> MAEKSIFNEPDVDFHLKLNQQLFHIPYELLSKRIKHTQAVINKETKSLHEHTAALNQIFEHNDVEHDELALAKITEMIRKVDHIERFLNTQIKSYCQILNRIKKRLEFFHELKDIKSQNSGTSHNGNNEGTRTKLIQWYQSYTNILIGDYLTRNNPIKYNSETKDHWNSGVVFLKQSQLDDLIDYDVLLEANRISTSLLHERNLLPLISWINENKKTLTKKSSILEFQARLQEYIELLKVDNYTDAIVCFQRFLLPFVKSNFTDLKLASGLLIFIKYCNDQKPTSSTSSGFDTEEIKSQSLPMKKDRIFQHFFHKSLPRITSKPAVNTTDYDKSSLINLQSGDFERYLNLLDDQRWSVLNDLFLSDFYSMYGISQNDPLLIYLSLGISSLKTRDCLHPSDDENGNQETETATTAEKEVEDLQLFTLHSLKRXXXXXXXXXXXXXXXXXXXXXXXXXXXX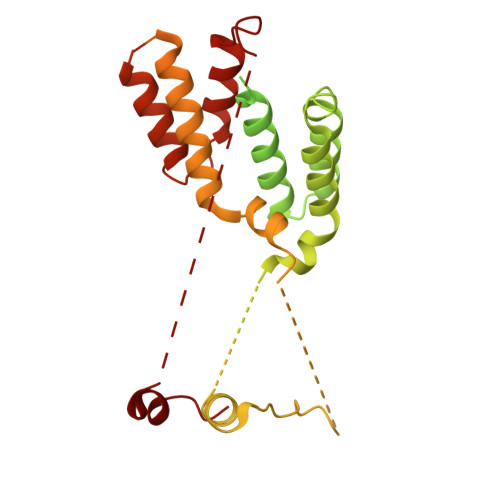XXXXXXXXXXXXXXXXXXXX>[2x]MAHHHHHHKKPINVAIFGSTGSIGTNALNIIRECNKIENVFNVKALYVNKSVNELYEQAREFLPEYLCIHDKSVYEELKELVKNIKDYKPIILCGDEGMKEICSSNSIDKIVIGIDSFQGL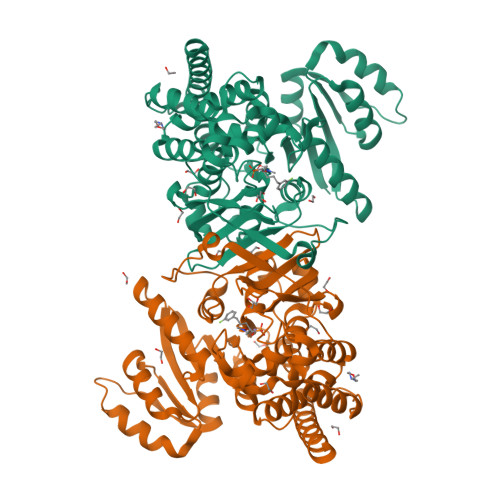YSTMYAIMNNKIVALANKESIVSAGFFLKKLLNIHKNAKIIPVDSEHSAIFQCLDNNKVLKTKCLQDNFSKINNINKIFLCSSGGPFQNLTMDELKNVTSENALKHPKWKMGKKITIDSATMMNKGLEVIETHFLFDVDYNDIEVIVHKECIIHSCVEFIDKSVISQMYYPDMQIPILYSLTWPDRIKTNLKPLDLAQVSTLTFHKPSLEHFPCIKLAYQAGIKGNFYPTVLNASNEIANNLFLNNKIKYFDISSIISQVLESFNSQKVSENSEDLMKQILQIHSWAKDKATDIYNKHNSS>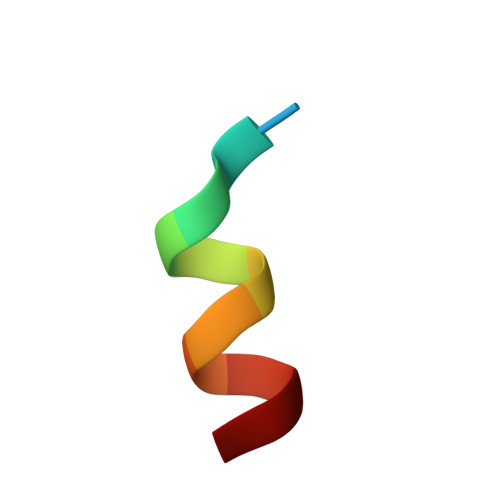 KENALLRYLLDK> MKLTPKELDKLMLHYAGELAKKRKEKGIKLNYVEAVALISAHIMEEARAGKKTAAELMQEGRTLLKPDDVMDGVASMIHEVGIEAMFPDGTKLVTVHTPIEANGKLVPGELFLKNEDITINEGKKAVSVKVKNVGDRPVQIGSHFHFFEVNRCLDFDREKTFGKRLDIASGTAVRFEPGEEKSVELIDIGGNRRIFGFNALVDRQADNESKKIALHRAKERG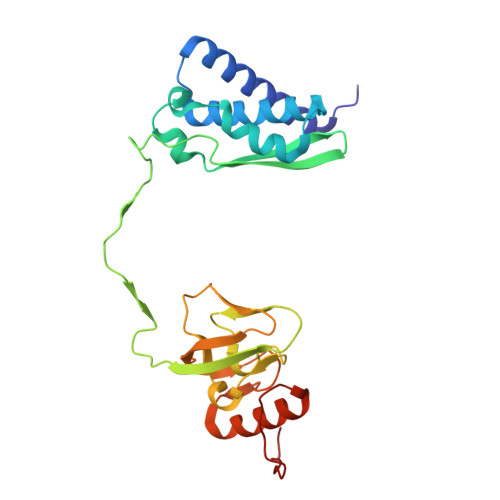FHGAKSDDNYVKTIKE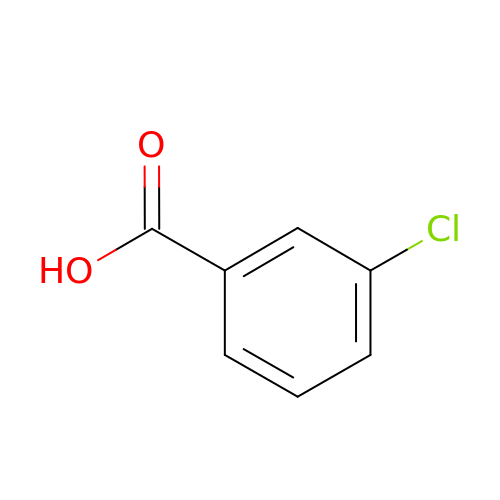3-chlorobenzoate | C7 H5 Cl O2 | LULAYUGMBFYYEX-UHFFFAOYSA-N>[2x]MKNTTTYDYIVVGGGTSGLVVANRLSENPDVSVLLLEAGASVFNNPDVTNANGYGLAFGSAIDWQYQSINQSYAGGKQQVLRAGKALGGTSTINGMAYTRAEDVQIDVWQKLGNEGWT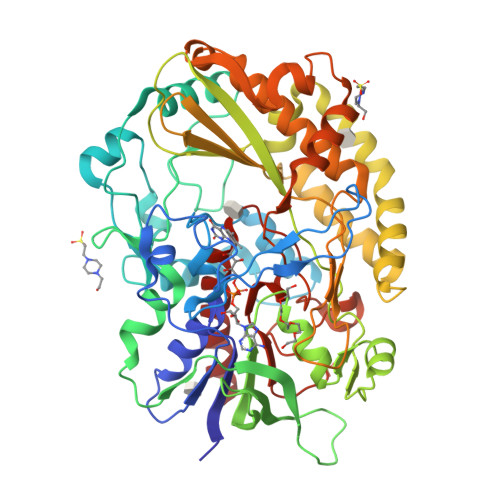WKDLLPYYLKSENLTAPTSSQVAAGAAYNPAVNGKEGPLKVGWSGSLASGNLSVALNRTFQAAGVPWVEDVNGGKMRGFNIYPSTLDVDLNVREDAARAYYFPYDDRKNLHLLENTTANRLFWKNGSAEEAIADGVEITSADGKVTRVHAKKEVIISAGALRSPLILELSGVGNPTILKKNNITPRVDLPTVGENLQDQFNNGMAGEGYGVLAGASTVTYPSISDVFGNETDSIVASLRSQLSDYAAATVKVSNGHMKQEDLERLYQLQFDLIVKDKVPIAEILFHPGGGNAVSSEFWGLLPFARGNIHISSNDPTAPAAINPNYFMFEWDGKSQAGIAKYIRKILRSAPLNKLIAKETKPGLSEIPATAADEKWVEWLKANYRSNFHPVGTAAMMPRSIGGVVDNRLRVYGTSNVRVVDASVLPFQVCGHLVSTLYAVAERASDLIKEDAKSA>AAPKDHLIHNHHKHEHAHAEHLGGSAWSHPQFEKGSGLEVLFQGPAEFASSQGNDKAPKNLHLVKRNAIKTRPSDALGGLEPGDPAPAFQVHTLDGMFVYSPRNESGRALIVHAFTNKSAFLECLWTWSESLSDLLDYLPSSTEVLMLSMDETAEQDALWMREQVYRAAAHRGKEILSRLHFSPTHVYNLGNWIPRVLYSWGCGGHNCGLGQVVFSSPDWKGPVIGKRLNARYDWLYAHWSTDPYRLLDVGDGCAPVASLKGAVAWVSEGGCSFFTKIKNMEKSNATGVLVYALPGNNIQDMNCKGDECFTSLHIPASMVHFQPKVKEALQKGRPVNVKFQVTPSRSFFFGIDQRGVLSEMGWFLYPSFRFMAWQAQWFVFNDALLEQLSQPAVTVSVFDHHDMHGNAGAHAVVDLPADISPYDVLELDTSLSCPGRRDETCAHWDHTVQLFVCCNDSSPYCNQELGRWVTAFRRGTGHWLTDVSPLIPLLNNKKCSFTMKTAPWAMPWMTTLNLRFSQSNKTERLYPFEVMPLFNGGTFDKDYNRRYHEITFSIPAATKKVELYAVITGHGSDDNNCGEFCVTSH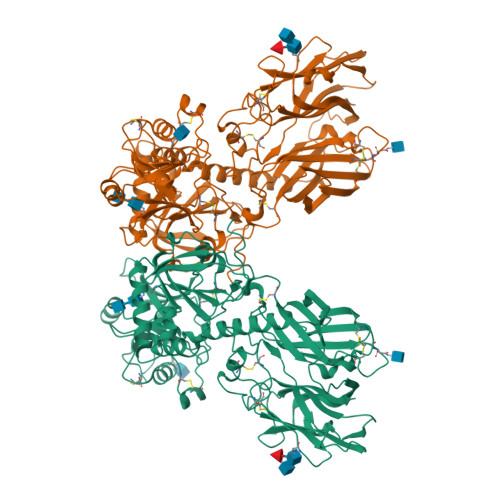YFLINRSINNTLVFEAAGSPLGCSLLVPKGGVPNECGTWLYGRGGWCDGLQVDPWRRDITSQLDMSGSNSVRYFGLFEGRDPNPKTDPGNILMYSYLVFYQ[2x]The complex consists of a tripartite ring comprising SMC1, SMC3, and RAD21 (also called SCC1 or Mcd1), which associates with a conserved peripheral fourth subunit that, in human somatic cells, is represented by two paralogs of the Scc3/STAG protein family, STAG1 or STAG2. STAG1/2 HEAT repeat proteins bind to the RAD21 subunit of the core cohesin ring and are required for the dynamic association of the complex with chromatin. The STAG1 protein is composed of HEAT repeats, a tandem repeat structural motif composed of two α helices linked by a short loop. STAG1 and STAG2, therefore, function redundantly in somatic mammalian cells to mediate sister chromatid cohesion, an event essential for cell viability during proliferation.

We have designed constructs of STAG1’s N-terminal and central region encompassing interaction regions I and II, and IV, respectively, and obtained crystal structures in both the presence and absence of the corresponding RAD21 peptides. We determined the structures of the N-terminal region of human STAG1, encompassing residues 86–420, in the absence and presence of a RAD21 peptide to 2.0 and 2.4 Å, respectively. As expected based on the degree of sequence homology (73% identities over equivalent regions), the structure is highly similar to STAG2 (∼1.3 Å RMSD).

>[4x]SMGGTLFEVVKLGKSAMQSVVDDWIESYKQDRDIALLDLINFFIQCSGCRGTVRIEMFRNMQNAEIIRKMTEEFDEDSGDYPLTMPGPQWKKFRSNFCEFIGVLIRQCQYSIIYDEYMMDTVISLLTGLSDSQVRAFRHTSTLAAMKLMTALVNVALNLSIHQDNTQRQYEAERNKMIGKRANERLELLLQKRKELQENQDEIENMMNSIFKGIFVHRYRDAIAEIRAICIEEIGVWMKMYSDAFLNDSYLKYVGWTLHDRQGEVRLKCLKALQSLYTNRELFPKLELFTNRFKDRIVSMTLDKEYDVAVEAIRLVTLILHGSEEALSNEDCENVYHLV>[2x]KFNDTLFGEMLHGYNNRTQHVNQGQVFQMTFRENNFIKDFPQLADGLLVIPLPVEEQCRGVLSEPLPDLQLLTGDIRYDEAMGYPMVQQWRVRSNLYRVKLSTITLAAGFTNVLKILTKESSREELLSFIQHYGSHYIAEALYGSELTCIIHFPSKKVQQQLWLQYQKETTELGSKKELKSMPFITYLSGLLTAQMLSDDQLISGVEIRCEEKGRCPSTCHLCRRPGKEQLSPTPVLLEINRVVPLYTLIQDNGTKEAFKSALMSS

Our focus here is on a PLP especially identified as being involved in neurodevelopment, astrotacin-2 (ASTN-2). ASTN-1 and ASTN-2 have been shown to interact directly with each other in vitro in a calcium-independent way with multiple regions of each protein apparently contributing to their interface. Both ASTN-1 and ASTN-2 are integral membrane proteins in which a large C-terminal domain (extracellular for ASTN-1, endosome luminal for ASTN-2) is complemented by an N-terminal cytosolic domain suspended between two transmembrane α-helices. Thus, the endosomal regions of ASTN-2 comprise a smaller N-terminal domain and a larger C-terminal domain whose structure we report here and which we refer to as its endodomain. We describe its unique combination of a canonical MACPF/CDC domain with a minimal epidermal growth factor (EGF)-like repeat (EGF-4), a previously unobserved type of fibronectin type III (Fn(III)) domain in which an additional two β-strands are folded across the core, and an annexin-like domain.

The N-terminus of the endodomain structure is formed by the canonical MACPF domain consisting of a central, broken, antiparallel four-stranded β-sheet that possesses a distinctive central approximately 90° bend. The most distinctive features of MACPF/CDC domains are two loops containing α-helices which link the core domain β-strands and which undergo refolding in pore-forming family members to generate a partial or complete β-barrel inserted in the membrane. In ASTN-2, the first such loop (loop 1, linking strands β1–β3 and β4–β5), comprises 19 residues and contains a single-turn 310-helix (η1) and which packs against the Fn(III) domain interface (see below; see electronic supplementary material, figure S5 for sequence alignment and secondary structure). The movement of ASTN-2 through the endolysosomal system suggests that its activity might be regulated by pH. We have determined structures of the endodomain at pH 7.5 and pH 5 and of the MACPF/CDC domain alone at pH 4, and find the regions of ASTN-2 resolved to be remarkably insensitive to acidification. In an attempt to investigate the effect of reduced pH on the ASTN-2 structure, we obtained crystals of constructs consisting of EGF-3 to the C-terminus (residues 649–1288) at pH 5 and of EGF-3 plus the MACPF domain at pH 4 (residues 649–984), though in neither case was EGF-3 resolved in the resulting structures. For crystallization of ASTN-2649-984, the protein was concentrated to 15 mg ml−1 and crystallized in 0.1 M citric buffer, pH 4.0–4.5, 20% PEG 1000. The crystal structure of the MACPF domain C-terminus at pH 5 and of the MACPF domain alone at pH 4 were solved by molecular replacement using copy A of the structure solved at pH 7.5 in PHASER and refinement was carried out in PHENIX. The conformations of the lower pH forms of ASTN-2 are very similar to the equivalent regions of the neutral pH structure (RMSDs 0.23 Å (pH 5) and 1.52 Å (pH 4)).>[4x]GSMKKERVITEFWDGKIIMVSPDDPKYALKKAEEVRELVDSELGFQQVSLRCPSQTRTYMFVSNEKKIVGCLIAEPIREAYRVLAEPPSLHSLHGEPLERHRAWRCSTEPEPAICGISRIWVFALMRRKAIASRMVDAVRSSFMYGSVLTTEEIAFSDPTPDGKLFASTYCKVPDFLVYNFVS;>[4x]RRVIGAKKDQYFL

Cohesin is loaded onto chromatin by the Scc2-Scc4 loader complex, however persistent cohesion cannot be established without the acetylation of two conserved tandem lysines on the Smc3 subunit by the Eco1 acetyltransferase (ACT). Eco1 is an acetyltransferase that belongs to the Gcn5-related N-acetyltransferase (GNAT) family. The xEco2 ACT fold is divided into two domains: the N-terminal domain contains α helix 1 and 2, and β strand 1–5 with a conserved central β hairpin insertion between β4 and β5 that is unique to cohesin ACTs; the C-terminal domain contains α helix 3, and β strand 6 and 7. The binding site for CoA is sandwiched between the N- and C-terminal domains involving β5 and α3, while the substrate peptides binds mainly to the central β hairpin and the C-terminal domain including the conserved C-terminal extension (C extension).

Next we investigated the slower but biologically more important K106 acetylation of Smc38, which is represented by our xEco2-K106-CoA structure. The substrate peptide adopts an extended β conformation different from K105-CoA binding but is accommodated by a conserved surface groove created by the same structural elements on xEco2 including the C-terminal loop of α1, the loop connecting β6 to α3, and the central β hairpin. Instead of the C extension, the binding of the K106 substrate peptide to xEco2 is mediated by main chain-side chain interactions through the formation of a parallel β sheet with the second strand of the central β hairpin. The side chain of the K106-CoA conjugate protrudes from a central CoA-binding cavity gated by the conserved L562 and F564 residues, whose hydrophobic side chains also contact the methylene groups of K105 at position -1 (P − 1) and the methyl group of A104 at P − 2. At P + 1 from the acetylated lysine, the acidic side chain of D107 forms a salt bridge with the indole side chain of W623 on the central β hairpin. The structure rationalizes the propensity of Eco1 substrates to have an aliphatic residue at P − 1 and P − 2, and an acidic/polar residue at P + 1 flanking the target lysine in our substrate motif consensus. However, in our xEco2-peptide K106 structure the Smc3 D107 interacts with the conserved R621 and W623 of xEco2 on the opposite side of the ε-amino group of the target lysine. The binding of the K106-CoA peptide is accompanied by an outward tilt of the central β hairpin from its peptide-free conformation with W623 displaced from a central hydrophobic pocket by Y109 of the K106 peptide. The binding of peptide K106-CoA forces a 180° flip of the C extension, exposing the entire length of the substrate-binding groove.Strigolactones (SLs) are phytohormones that control many aspects of plant growth. Despite their relatively recent discovery as plant hormones, rapid progress has been made in understanding SL function, including the identification of a signalling pathway for SLs. This pathway involves the SL receptors of the DWARF14 (D14) class of α/β-hydrolase enzymes, the MORE AXILLARY GROWTH2 (MAX2) F-box proteins, and the SUPPRESSOR OF MAX2 1 (SMAX1) and SMAX1-LIKE (SMXL) family of chaperonin-like proteins. The D14 α/β-hydrolase enzyme uses a Ser–His–Asp catalytic triad to perceive and hydrolyse SLs simultaneously. OsD14 has a α/β-hydrolase fold with a seven-stranded β-sheet core domain flanked by seven α-helices, of which two are shorter 310-helices.

The structure of O. sativa Dwarf14 (OsD14) was determined by X-ray crystallography to a resolution of 1.35 Å from a construct lacking the first 51 residues. Inserted between strands five and six of the central sheet are four helices connected to the core by a β-hairpin loop on its N-terminal side and a shorter loop on the other side. This domain, commonly named the helical cap, forms a V-shaped lid over a deep cavity, which is assumed to bind the SL hormone. At the bottom of the cavity is a canonical catalytic triad consisting of Ser147, His297, and Asp268. After model building of the protein, residual density was observed in the ligand-binding cavity. We identified this as originating from MPD, which was used as a precipitating agent during crystallization. MPD was added as a racemic mixture of (4S)-2-methyl-2,4-pentanediol and (4R)-2-methyl-2,4-pentanediol, and it appears that both stereoisomers were able to bind in the cavity. Judging from the electron density, there was a preference for binding the 4S stereoisomer in one subunit (arbitrarily named molecule B in the PDB co-ordinate file). MPD is located some distance away from the catalytic triad, forms several hydrophobic interactions with residues lining the cavity (Phe78, Phe176, Phe186, Val194, Val244, and Phe245), and hydrogen-bonds to the hydroxyl oxygen of Tyr209 and to Oγ of Ser147 and Nε2 of His297 via a water molecule. In the second subunit (named molecule A), the binding of the 4R stereoisomer appears to be preferred, and the direct interaction with the Tyr209 hydroxyl group is replaced by a solvent-mediated contact. The helical cap covers MPD like a dome, but is open to solvent on one side in this conformational state of the receptor.

>[2x]SGAKLLQILNVRVVGSGERVVVLSHGFGTDQSAWSRVLPYLTRDHRVVLYDLVCAGSVNPDHFDFRRYDNLDAYVDDLLAILDALRIPRCAFVGHSVSAMIGILASIRRPDLFAKLVLIGASPRFLNDSDYHGGFELEEIQQVFDAMGANYSAWATGYAPLAVGADVPAAVQEFSRTLFNMRPDISLHVCQTVFKTDLRGVLGMVRAPCVVVQTTRDVSVPASVAAYLKAHLGGRTTVEFLQTEGHLPHLSAPSLLAQVLRRALARY> MVSSAQMGFNLQALLEQLSQDELSKFKYLITTFSLAHELQKIPHKEVDKADGKQLVEILTTHCDSYWVEMASLQVFEKMHRMDLSERAKDEVREAALKSFNKRKPLSLGITRKERPPLDVDEMLERFKTEAQAFTETKGNVICLGKEVFKGKKPDKDNRCRYILKTKFREMWKSWPGDSKEVQVMAERYKMLIPFSNPRVLPGPFSYTVVLYGPAGLGKTTLAQKLMLDWAEDNLIHKFKYAFYLSCRELSRLGPCSFAELVFRDWPELQDDIPHILAQARKILFVIDGFDELGAAPGALIEDICGDWEKKKPVPVLLGSLLNRVMLPKAALLVTTRPRALRDLRILAEEPIYIRVEGFLEEDRRAYFLRHFGDEDQAMRAFELMRSNAALFQLGSAPAVCWIVCTTLKLQMEKGEDPVPTCLTRTGLFLRFLCSRFPQGAQLRGALRTLSLLAAQGLWAQTSVLHREDLERLGVQESDLRLFLDGDILRQDRVSKGCYSFIHLSFQQFLTALFYTLEKEEEEDRDGHTWDIGDVQKLLSGVERLRNPDLIQAGYYSFGLANEKRAKELEATFGCRMSPDIKQELLRCDISCKGGHSTVTDLQELLGCLYESQEEELVKEVMAQFKEISLHLNAVDVVPSSF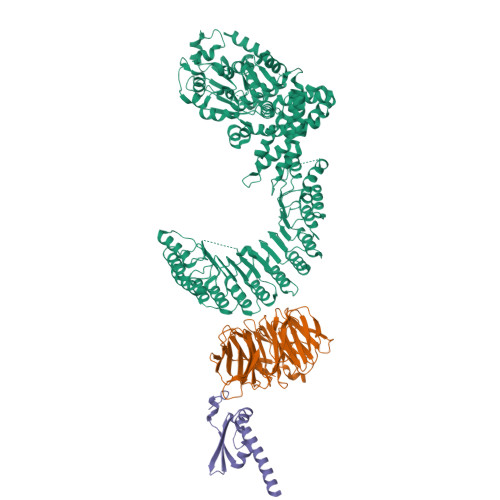CVKHCRNLQKMSLQVIKENLPENVTASESDAEVERSQDDQHMLPFWTDLCSIFGSNKDLMGLAINDSFLSASLVRILCEQIASDTCHLQRVVFKNISPADAHRNLCLALRGHKTVTYLTLQGNDQDDMFPALCEVLRHPECNLRYLGLVSCSATTQQWADLSLALEVNQSLTCVNLSDNELLDEGAKLLYTTLRHPKCFLQRLSLENCHLTEANCKDLAAVLVVSRELTHLCLAKNPIGNTGVKFLCEGLRYPECKLQTLVLWNCDITSDGCCDLTKLLQEKSSLLCLDLGLNHIGVKGMKFLCEALRKPLCNLRCLWLWGCSIPPFSCEDLCSALSCNQSLVTLDLGQNPLGSSGVKMLFETLTCSSGTLRTLRLKIDDFNDELNKLLEEIEEKNPQLIIDTEKHHPWAERPSSHDFMI;> MTSRDQPRPKGPPKSTSPCPGISNSESSPTLNYQGILNRLKQFPRFSPHFAAELESIYYSLHKIQQDVAEHHKQIGNVLQIVESCSQLQGFQSEEVSPAEPASPGTPQQVKDKTLQESSFEDIMATRSSDWLRRPLGEDNQPETQLFWDKEPWFWHDTLTEQLWRIFAGVHDEKAKPRDRQQAPGLGQESKAPGSCDPGTDPCPEDASTPRPPEASSSPPEGSQDRNTSWGVVQEPPGRASRFLQSISWDPEDFEDAWKRPDALPGQSKRLAVPCKLEKMRILAHGELVLATAISSFTRHVFTCGRRGIKVWSLTGQVAEDRFPESHLPIQTPGAFLRTCLLSSNSRSLLTGGYNLASVSVWDLAAPSLHVKEQLPCAGLNCQALDANLDANLAFASFTSGVVRIWDLRDQSVVRDLKGYPDGVKSIVVKGYNIWTGGPDACLRCWDQRTIMKPLEYQFKSQIMSLSHSPQEDWVLLGMANGQQWLQSTSGSQRHMVGQKDSVILSVKFSPFGQWWASVGMDDFLGVYSMPAGTKVFEVPEMSPVTCCDVSSNNRLVVTGSGEHASVYQITY;> MVDDAGAAESQRGKQTPAHSLEQLRRLPLPPPQIRIRPWWFPVQELRDPLVFYLEAWLADELFGPDRAIIPEMEWTSQALLTVDIVDSGNLVEITVFGRPRVQNRVKSMLLCLAWFHREHRARAEKMKHLEKNLKAHASDPHSPQDPVA> GSHMPKRTFTKEDIRKFAEEENVRYLRLQFTDILGTIKNVEVPVSQLEKVLDNEMMFDGSSIEGFVRIEESDMYLHPDLDTWVIFPWTAGQGKVARLIC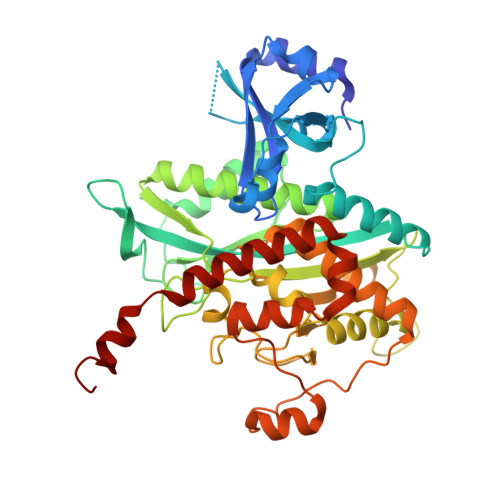DVYKTDGTPFEGDPRANLKRVLKEMEDLGFTDFNLGPEPEFFLFKLDEKGEPTLELNDDGGYFDLAPTDLGENCRRDIVLELEDMGFDIEASHHEVAPGQHEIDFKYADAVTACDNIQTFKLVVKTIARKHNLHATFMPKPLFGVNGSGMHFNVSLFKGKENAFFDPNTEMGLTETAYQFTAGVLKNARGFTAVCNPLVNSYKRLVPGYEAPCYIAWSGKNRSPLIRVPSSRGLSTRIEVRSVDPAANPYMALAAILEAGLDGIKNKLKVPEPVNQNIYEMNREEREAVGIQDLPSTLYTALKAMRENEVIKKALGNHIYNQFINSKSIEWDYYRTQVSEWERDQYMKQY>[2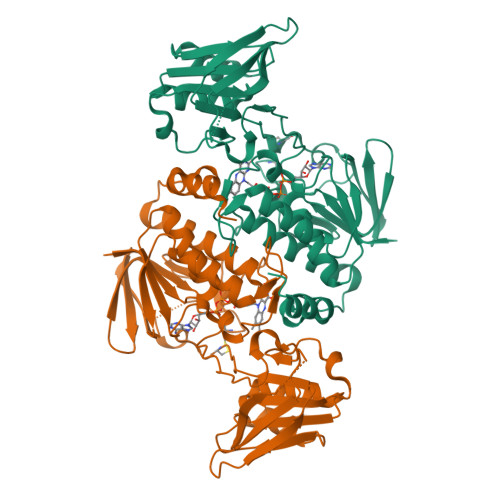x]MKDVTIIGGGPSGLYASFYAGLRDMSVRLIDVQSELGGKMRIYPEKIIWDIGGIAPKPCHEILKDTIKQGLYFKPEVHLNERVVDIRKKAERHFEVETEAGEIYTSKAVIIAIGAGIINPKQLDVKGVERYQLTNLHYVVQSYRRFKDKDVLISGGGNTALDWAHDIAKIAKSVTVVYRKEDVSGHEAMKTLVTDLNVKLCPKTRIKYLVGNDDETHISEVVLEHVESGDRHTVKFDDVIISHGFDRCNTLLSETSSKLDMHDDCRVKGFGNTTTSIPGIYACGDIVYHDAKSHLIASAFSDGANAANLAKTYIQPDANAEGYVSSHHEVFKEANKTIVNKHLY>[2x]GSFTFSPGQDIQLIPPLINLLMSIEPDVIYAGHDNTKPDTSSSLLTSLNQLGERQLLSVVKWSKSLPGFRNLHIDDQITLIQYSWMSLMVFGLGWRSYKHVSGQMLYFAPDLILNEQRMKESSFYSLCLTMWQIPQEFVKLQVSQEEFLCMKVLLLLNTIPLEGLRSQTQFEEMRSSYIRELIKAIGLRQKGVVSSSQRFYQLTK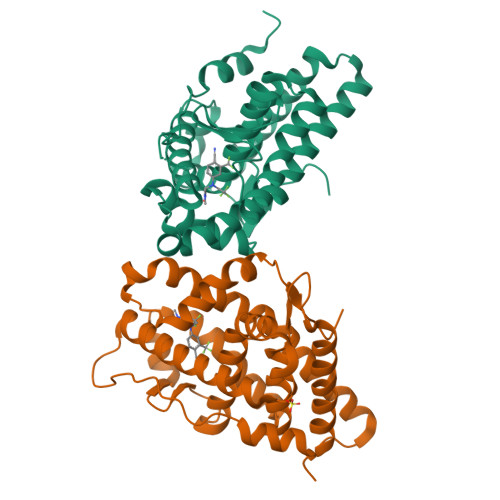LLDNLHDLVKQLHLYCLNTFIQSRALSVEFPEMMSEVIAAQLPKILAGMVKPLLFHKK>GPHMSDHKFLTQAVEEAYKGVDCGDGGPFGAVIVHNNEVVASCHNMVLKYTDPTAHAEVTAIREACKKLNKIELSECEIYASCEPCPMCFGAIHLSRLKRLVYGAKAEAAIAIGFDDFIADALRGTGVYQKSSLEIKKADGNGAAIAEQVFQNTKEKFRLY[2x]

In plants, guanosine deaminase (GSDA) catalyzes the deamination of guanosine for nitrogen recycling and re-utilization. The other involves the hydrolysis of Gua to guanine (G), followed by its deamination to xanthine under the action of guanine deaminase (GDA). Both deaminases are zinc-dependent enzymes, which rely on a catalytic water molecule to attack the amino group-connecting C2 atom to proceed with the catalysis. The zinc ions are tightly bound to the active site, coordinated by the completely conserved residues His80, Cys113, Cys110, and the key water molecule. AtGSDA catalysis needs two key sub-processes: the activation of water and re-capping of the active site, which proceed via the two critical residues Glu82 and Tyr185, respectively.

As a reference, we first cocrystallized the natural substrate Gua with the WT enzyme. The quick soaking process (within 2 min) resulted in the complete deamination. Specifically, the essential C-terminal loops of the enzyme would re-cap the active site by forming the key contact with N7 of Gua via the side chain of Tyr185. However, it was not difficult to tell that Xan stabilizes the enzyme more than Gua.Fatty acid synthase (FASN) catalyzes the de novo synthesis of palmitate, a 16-carbon chain fatty acid that is the primary precursor of lipid metabolism and an important intracellular signaling molecule. In contrast, Type I FAS found in eukaryotes and some actinobacteria are large complexes of multi-domain protomers that are composed of one or two repeating polypeptides that are each encoded by a single gene and organized in a symmetric or pseudo-symmetric assembly. In humans, the FASN gene encodes a 273 kDa polypeptide that comprises the catalytic domains necessary for palmitate synthesis, which further homodimerizes into a pseudo-symmetric complex. The contact point of the condensing and modifying regions is the neck region, a flexible linker composed of two short unstructured loops which allow for continuous swinging and swiveling motions of the two regions relative to each other, maximizing ACP accessibility to all catalytic centers. hFASN is a validated anti-cancer target and is over-expressed in solid tumors including those from breast, prostate, liver, and lung tissues.

For this effort, we selected Denifanstat, an orally bioactive molecule with antineoplastic activity. Denifanstat (TVB-2640) blocks consumption of NADPH by the KR domain in both protein preparations. We found that the drug binds the same pocket and interacts predominantly with catalytic residues from the KR domain and the nicotinamide of NADPH. However, the binding conformation of Denifanstat is different from triazolone and piperazine compounds, with the Denifanstat being more solvent exposed and interacting with residues from the dynamic loop predicted to be involved in ACP binding. To the best of our knowledge, this is the first cryoEM model of hFASN complexed with the first-in-class anti-neoplastic inhibitor that is undergoing clinical trials and can be used as a platform for rational design of other novel hFASN inhibitors. Finally, we solved the structure of this region bound to an anti-cancer drug, Denifanstat (i.e., TVB-2640), demonstrating the utility of our approach as a platform for structure guided design of future hFASN small molecule inhibitors.

>[2x]GGSPSAAIYNIDTSSESPDHYLVDHTLDGRVLFPATGYLSIVWKTLARALGLGVEQLPVVFEDVVLHQATILPKTGTVSLEVRLLEASRAFEVSENGNLVVSGKVYQWDDPDPRLFDHPESPTPNPTEPLFLAQAEVYKELRLRGYDYGPHFQGILEASLEGDSGRLLWKDNWVSFMDTMLQMSILGSAKHGLYLPTRVTAIHIDPATHRQKLYTLQDKAQVADVVVSRWLRVTVAGGVHISGLHTESAPRRQQEQQVPILEKFCFTPHTEEGCLSERAALQEELQLCKGLVQALQTKVTQQGLKMVVPGLDGAQIPRDPSQQELPRLLSAACRLQLNGNLQLELAQVLAQERPKLPEDPLLSGLLDSPALKACLDTAVENMPSLKMKVVEVLAGHGHLYSRIPGLLSPHPLLQLSYTATDRHPQALEAAQAELQQHDVAQGQWDPADPAPSALGSADLLVCNCAVAALGDPASALSNMVAALREGGFLLLHTLLRGHPLGDIVAFLTSTEPQYGQGILSQDAWESLFSRVSLRLVGLKKSFYGSTLFLCRRPTPQDSPIFLPVDDTSFRWVESLKGILADEDSSRPVWLKAINCATSGVVGLVNCLRREPGGNRLRCVLLSNLSSTSHVPEVDPGSAELQKVLQGDLVMNVYRDGAWGAFRHFLLEEDKPEEPTAHAFVSTLTRGDLSSIRWVCSSLRHAQPTCPGAQLCTVYYASLNFRDIMLATGKLSPDAIPGKWTSQDSLLGMEFSGRDASGKRVMGLVPAKGLATSVLLSPDFLWDVPSNWTLEEAASVPVVYSTAYYALVVRGRVRPGETLLIHSGSGGVGQAAIAIALSLGCRVFTTVGSAEKRAYLQARFPQLDSTSFANSRDTSFEQHVLWHTGGKGVDLVLNSLAEEKLQASVRCLATHGRFLEIGKFDLSQNHPLGMAIFLKNVTFHGVLLDAFFNESSADWREVWALVQAGIRDGVVRPLKCTVFHGAQVEDAFRYMAQGKHIGKVVVQVLAEEPEAVLKGAKPKLMSAISKTFCPAHKSYIIAGGLGGFGLELAQWLIQRGVQKLVLTSRSGIRTGYQAKQVRRWRRQGVQVQVSTSNISSLEGARGLIAEAAQLGPVGGVFNLAVVLRDGLLENQTPEFFQDVCKPKYSGTLNLDRVTREACPELDYFVVFSSVSCGRGNAGQSNYGFANSAMERICEKRRHEGLPGLAVQWGAIGDVGILVETMSTNDTIVSGTLPQRMASCLEVLDLFLNQPHMVLSSFVLAEKAAAYRDRDSQRDLVEAVAHILGIRDLAAVNLDSSLADLGLDSLMSVEVRQTLERELNLVLSVREVRQLTLRKLQELSSKADEASELACPTPKEDGLAQQQTQLNLRSLLVNPEGPTLMRLNSVQSSERPLFLVHPIEGSTTVFHSLASRLSIPTYGLQCTRAAPLDSIHSLAAYYIDCIRQVQPEGPYRVAGYSYGACVAFEMCSQLQAQQSPAPTHNSLFLFDGSPTYVLAYTQSYRAKLTPGCEAEAETEAICFFVQQFTDMEHNRVLEALLPLKGLEERVAAAVDLIIKSHQGLDRQELSFAARSFYYKLRAAEQYTPKAKYHGNVMLLRAKTGGAYGEDLGADYNLSQVCDGKVSVHVIEGDHRTLLEGSGLESIISIIHSSLAEPRVSVREGLESRGPHHHHHH(3~{R},4~{R})-4-(3,4-dihydro-1~{H}-isoquinolin-2-yl)pyrrolidin-3-ol | C13 H18 N2 O | 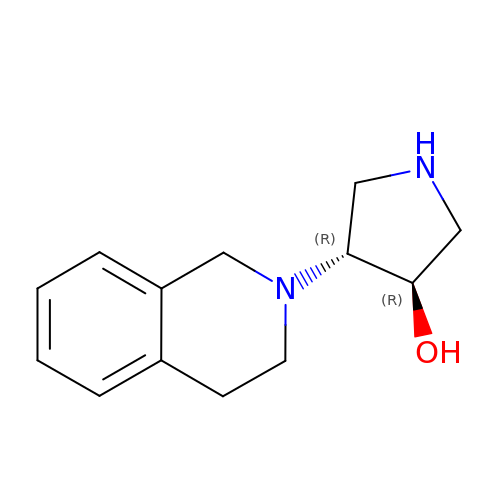YOMLWJZQKDDDDV-CHWSQXEVSA-N> MKIMQVEKTLVSTNRIADMGHKPLLVVWEKPGAPRQVAVDAIGCIPGDWVLCVGSSAAREAAGSKSYPSDLTIIGIIDQWNGE;>MAAVTGIALGMIETRGLVPAIEAADAMTKAAEVRLVGRQFVGGGYVTVLVRGETGAVNAAVRAGADACERVGDGLVAAHIIARVHSEVENILPKAPEA[8x];>[2x]MPFCTSTPEPEAQSTEQSLTCEGQIISGTSVDASDLVTGNEIGEQQLISGDAYVGAQQTGCLPTSPRFNQTGNVQSMGFKNTNQPEQNFAPGEVMPTDFSIQTPARSAQNRITGNDIAPSGRITGPGMLATGLITGTPEFRHAARELVGSPQPMAMAMANRNKAAQAPVVQPEVVATQEKPELVCAPRSDQMDRVSGEGKERCHITGDDWSVNKHITGTAGQWASGRNPSMRGNARVVETSAFANRNVPKPEKPGSKITGSSGNDTQGSLITYSGGARG

Among diverse BMCs, carboxysomes are specific CO2-fixing BMCs found in all cyanobacteria and many proteobacteria. The carboxysome uses a polyhedral protein shell to encapsulate the key CO2 fixation enzymes, ribulose-1,5-bisphosphate carboxylase/oxygenase (Rubisco) and carbonic anhydrase (CA). Carboxysome shells are typically composed of three groups of structural components that form hexamers, pentamers, and trimers. Here, we generated recombinant α-carboxysome shells of Halothiobacillus neapolitanus by expressing all the shell proteins (involving three CsoS1 hexameric proteins and two CsoS4 pentameric proteins), together with the C-terminal domain of CsoS2 (CsoS2-C) that mediates shell assembly.

CsoS1A and CsoS1C differ by only two amino acids (3rd and 97th amino acids). The cryo-EM structure at 1.8-Å resolution showed that the resulting T = 9 shell resembles the T = 9 mini-shell formed by CsoS1A. Therefore, we speculate that CsoS1A and CsoS1C share similar features and can be naturally interchangeable during shell assembly. We confirmed that, similar to CsoS1A, CsoS1C can form a hexamer alone, while when coexpressed with CsoS1B, CsoS1C can form CsoS1C/B heterohexamers. Mini-shells (~25 nm, T = 3) can be formed in the presence of a single type of hexamer (CsoS1A or CsoS1C) and pentamer (CsoS4A).As a model β-strand mediated PPI, we use the GKAP/SHANK-PDZ50 which, plays a role in the organization of synaptic protein complexes and has been linked to several neuronal disorders. There are >250 PDZ domains with several therapeutically relevant proteins known to exhibit their function through a PDZ mediated interaction. Class I PDZ domains bind to consensus sequences with a Thr/Ser in the -2 position from the C-terminus, with the C-terminus hydrophobic residue and free carboxylate being the main determinants of affinity. Here, we used dynamic ligation screening to identify peptide-fragment hybrids linked through an acylhydrazone bond, that are able to functionally mimic a β-strand and inhibit its PPI using GKAP/SHANK1 PDZ as a model interaction.

Interestingly, the most potent hybrids formed from 3 and 4 contained the same carboxylic acid functionalized aromatic aldehyde fragments (A047 and A048), indicating that these types of fragments might play an important role in binding. In all hybrids, the hydrazone bond existed in an E configuration with the aromatic ring of the fragment co-planar with the hydrazone. Interestingly, hybrids with the C3 linker (compound 4 hydrazones) showed more favourable enthalpic contributions and slightly higher affinity in comparison to compounds having the C2 linker (compound 3) when the same fragment was attached. This indicated that the more flexible linker allows for a better orientation of the fragment leading to a more favourable enthalpy of binding, but also increases the entropic cost of binding, leading only to a moderate difference in the overall binding energy. We compared the ability to bind to SHANK1 PDZ against the ability to bind to the PDZ domain of PSD-95, a therapeutically important target in neuronal diseases and cancer. We monitored the binding using chemical shift perturbations in the 1H–15N HSQC spectra of the PDZ domain of PSD-95 (Tables S7 and S8†).

>[2x]GPLGSDYIIKEKTVLLQKKDSEGFGFVLRGAKAQTPIEEFTPTPAFPALQYLESVDEGGVAWRAGLRMGDFLIEVNGQNVVKVGHRQVVNMIRQGGNTLMVKVVMVTRHPDM> MSGSSAGSSFVHLHNHTEYSMLDGAAKITPMLAEVERLGMPAVGMTDHGNMFGASEFYNSATKAGIKPIIGVEAYIAPGSRFDTRRILWGDPSQKADDVSGSGSYTHLTMMAENATGLRNLFKLSSHASFEGQLSKWSRMDAELIAEHAEGIIITTGCPSGEVQTRLRLGQDREALEAAAKWREIVGPDNYFLELMDHGLTIERRVRDGLLEIGRALNIPPLATNDCHYVTRDAAHNHEALLCVQTGKTLSDPNRFKFDGDGYYLKSAAEMRQIWDDEVPGACDSTLLIAERVQSYADVWTPRDRMPVFPVPDGHDQASWLRHEVDAGLRRRFPAGPPDGYRERAAYEIDVICSKGFPSYFLIVADLISYARSAGIRVGPGRGSAAGSLVAYALGITDIDPIPHGLLFERFLNPERTSMPDIDIDFDDRRRGEMVRYAADKWGHDRVAQVITFGTIKTKAALKDSARIHYGQPGFAIADRITKALPPAIMAKDIPLSGITDPSHERYKEAAEVRGLIETDPDVRTIYQTARGLEGLIRNAGVHACAVIMSSEPLTEAIPLWKRPQDGAIITGWDYPACEAIGLLKMDFLGLRNLTIIGDAIDNVRANRG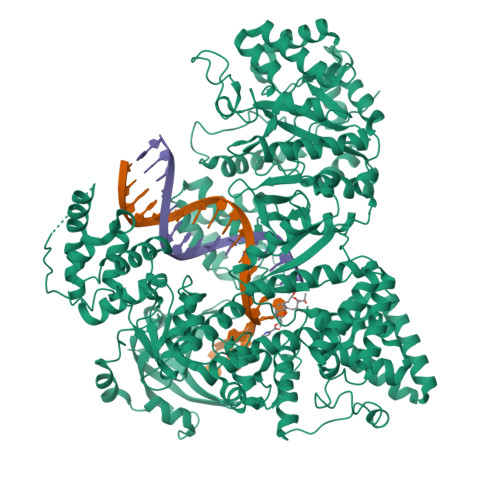IDLDLESVPLDDKATYELLGRGDTLGVFQLDGGPMRDLLRRMQPTGFEDVVAVIALYRPGPMGMNAHNDYADRKNNRQAIKPIHPELEEPLREILAETYGLIVYQEQIMRIAQKVASYSLARADILRKAMGKKKREVLEKEFEGFSDGMQANGFSPAAIKALWDTILPFADYAFNKSHAAGYGMVSYWTAYLKANYPAEYMAGLLTSVGDDKDKAAVYLADCRKLGITVLPPDVNESGLNFASVGQDIRYGLGAVRNVGANVVGSLLQTRNDKGKFTDFSDYLNKIDISACNKKVTESLIKAGAFDSLGHARKGLFLVHSDAVDSVLGTKKAEALGQFDLFGSNDDGTGTADPVFTIKVPDDEWEDKHKLALEREMLGLYVSGHPLNGVAHLLAAQVDTAIPAILDGDVPNDAQVRVGGILASVNRRVNKNGMPWASAQLEDLTGGIEVMFFPHTYSSYGADIVDDAVVLVNAKVAVRDDRIALIANDLTVPDFSNAEVERPLAVSLPTRQCTFDKVSALKQVLARHPGTSQVHLRLISGDRITTLALDQSLRVTPSPALMGDLKELLGPGCLGS> MELIKGQALFLELDKKDFLSLKNNDKNIPTFAHPKNQEKILAIFSLPYKNPPQNTKLIAFYKDKKEEIFIKTLEGNYKSEKLQVENKKIF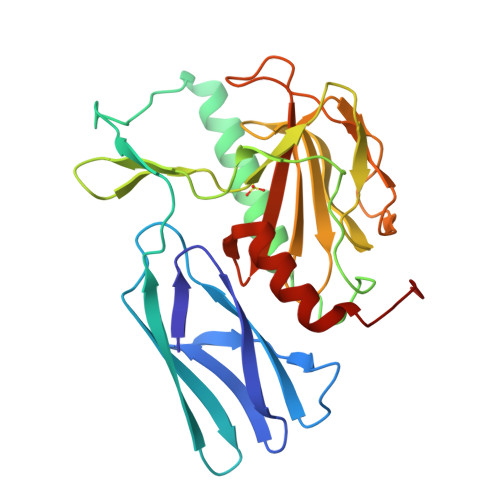PPKTIQERIAKELKEANAIYSSYTPKALFNGAFNIPLNSFITSDFGKARTFNEKVASYHSGTDFRAATGTPIYAANSGVVKIAKDRYFAGNSVVIDHGFGIYSQYYALSKIDVKVGQKIKKGELIGLSGASGRVSGPHLHFGILAGGKQVDPLDFVSKFNAIFQLEHHHHHH>MSRPAPLTLIGLGPMGQAMGNALLDRGHGLTVWNRTASRADALVERGAVRAPDVAAAVAANELVVLSLTDYDAMYALLGPAADALAGKVVVNLSSDTPEKTRAGARWIAEHGGTLIAGGVTVPPSGIGSPESSAFYSGPSAAFERHRETLRTLTRTDYRGEDPGL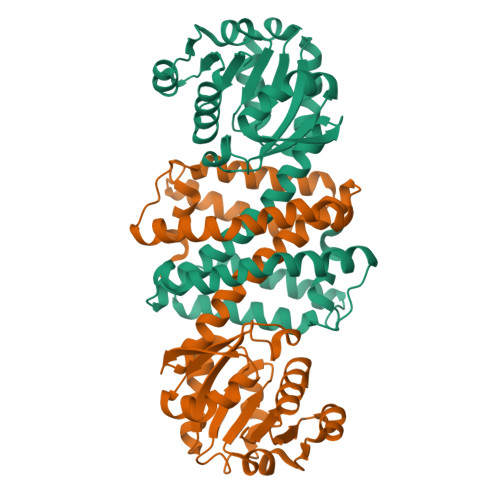AALMYQIGMVMFWNAMLGYWQAVALADANGLKAADILPHASDTVASLPGFLRFYADRIDTGHHGGDVDRLAMGTASVEHILHTMADSGVDTALPEAVVAFFRRGMAAGYAENSFSSMVELLKKPS[2x]>[4x]MASMTGGQQMGRGSDYFEPQQQQQQQQQQPQGASTPKVFVGYSIYKGKAALTVEPRSPEFSPLDSGAFKLSREGMVMLQFAPAAGVRQYDWS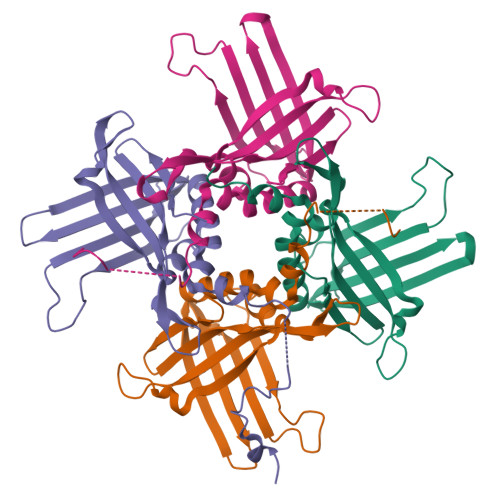RKQVFSLSVTEIGSIISLGTKDSCEFFHDPNKGRSDEGRVRKVLKVEPLPDGSGHFFNLSVQNKLINLDENIYIPVTKAEFAVLVSAFNFVMPYLLGWHTAVNSFKPEDASRSNNANPRSGAELEWNLEHHHHHH>AYTKISDVIVPELFNPYVINTTTQLSAFFQSGIAATDDELNALAKKAGGGSTLNMPYWNDLDGDSQVLNDTDDLVPQKINAGQDKAVLILRGNAWSSHDLAATLSGSDPMQAIGSRVAAYWAREMQKIVFAELAGVFSNDDMKDNKLDISGTADGIYSAETFVDASYKLGDHESLLTAIGMHSATMASAVKQDLIEFVKDSQSGIRFPTYMNKRVIVDDSMPVE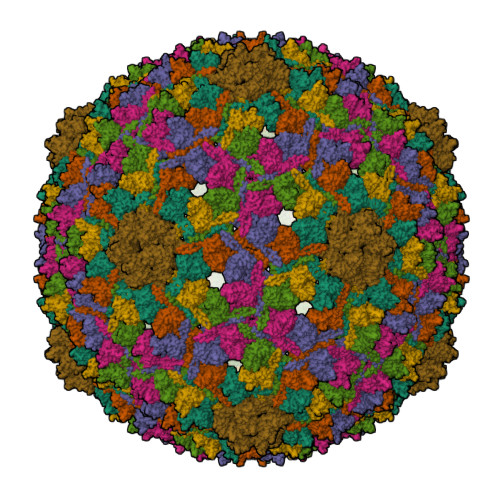TLEDGTKVFTSYLFGAGALGYAEGQPEVPTETARNALGSQDILINRKHFVLHPRGVKFTENAMAGTTPTDEELANGANWQRVYDPKKIRIVQFKHRLQA[7x]1-ALPHA-D-RIBOFURANOSYL-BENZIMIAZOLE-5'-PHOSPHATE | C12 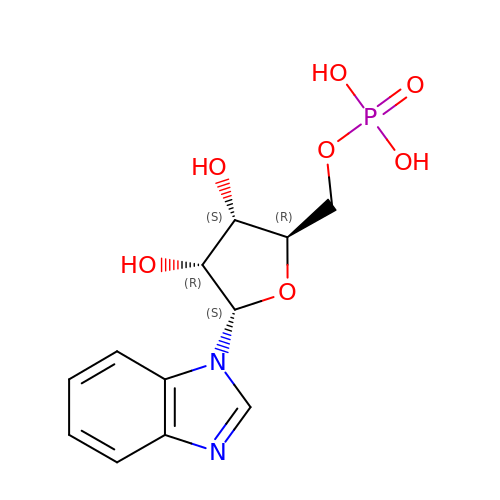H15 N2 O7 P | YPYFPLLZCVEYCS-KKOKHZNYSA-N> MFENITAAPADPILGLADLFRADERPGKINLGIGVYKDETGKTPVLTSVKKAEQYLLENETTKNYLGIDGIPEFGRCTQELLFGKGSALINDKRARTAQTPGGTGALRVAADFLAKNTSVKRVWVSNPSWPNHKSVFNSAGLEVREYAYYDAENHTLDFDALINSLNEAQAGDVVLFHGCCHNPTGIDPTLEQWQTLAQLSVEKGWLPLFDFAYQGFARGLEEDAEGLRAFAAMHKELIVASSYSKNFGLYNERV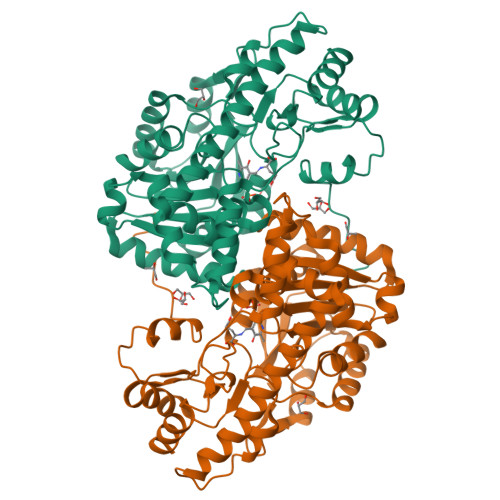GACTLVAADSETVDRAFSQMKAAIRANYSNPPAHGASVVATILSNDALRAIWEQELTDMRQRIQRMRQLFVNTLQEKGANRDFSFIIKQNGMFSFSGLTKEQVLRLREEFGVYAVASGRVNVAGMTPDNMAPLCEAIVAVL>MSQVKRANENRETARFIKKHKKQVTNPIDEKNGTSNCIVRVPIALYVSLAPMYLENPLQGVMKQHLNPLVMKYNNKVGGVVLGYEGLKILDADPLSKEDTSEKLIKITPDTPFGFTWCHVNLYVWQPQVGDVLEGYIFIQSASHIGLLIHDAFNASIKKNNIPVDWT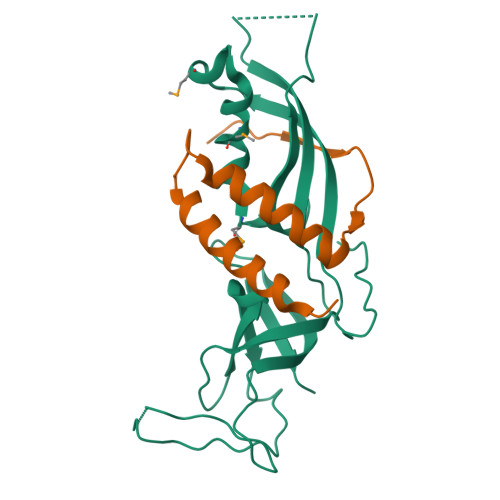FVHNDGNRSLGHWVDSNGEPIDGKLRFTVRNVHTTGRVVSVDGTLIS[3x];>MMKGSRRTGNNTATTLNTPVVIHATQLPQHVSTDEVLQFLESFIDEKENIIDIDTNLSSSISQLKRIQRDFKGLPPAQDFSAAPIQV[3x]> XGELAALKELAALKA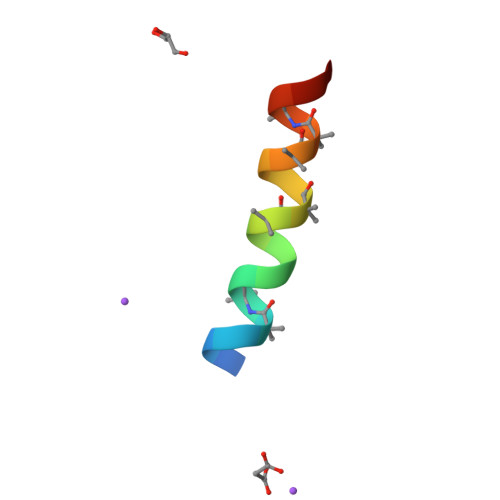AAWKGX>LMGCVAETPPRFTRTPVDQTGVSGGVASFICQATGDPRPKIVWNKKGKKVSNQRFEVIEFDDGSGSVLRIQPLRTPRDEAIYECVASNNVGEISVSTRLTVLREDQIPRGFPTIDMGPQLKVVERTRTATMLCAASGNPDPEITWFKDFLPVDTSNNNGRIKQLRSESIGGTPIRGALQIEQSEESDQGKYECVATNSAGTRYSAPANLYVRELREVRRVPPRFSIPPTNHEIMPGGSVNITCVAVGSPMPYVKWMLGAEDLTPEDDMPIGRNVLELNDVRQSANYTCVAMSTLGVIEAIAQITVKALPKPPGTPVVTESTATSITLTWDSGNPEPVSYYIIQHKPKNSEEPYKEIDGIATTRYSVAGLSPYSDYEFRVVAVNNIGRGPASEPVLTHHHHHH[2x];>QICPKRCVCQILSPNLATLCAKKGLLFVPPNIDRRTVELRLADNFVTNIKRKDFANMTSLVDLTLSRNTISFITPHAFADLRNLRALHLNSNRLTKITNDMFSGLSNLHHLILNNNQLTLISSTAFDDVFALEELDLSYNNLETIPWDAVEKMVSLHTLSLDHNMIDNIPKGTFSHLHKMTRLDVTSNKLQKLPPDPLFQRAQVLATSGIISPSTFALSFGGNPLHCNCELLWLRRLSREDDLETCASPPLLTGRYFWSIPEEEFLCEPPLITRHTHEMRVLEGQRATLRCKARGDPEPAIHWISPEGKLISNATRSLVYDNGTLDILITTVKDTGAFTCIASNPAGEATQIVDLHIIKLPHHHHHH[2x]

Type-IIa receptor protein tyrosine phosphatases (RPTPs) and neurexins are the two major presynaptic organizers. In mammals, the type-IIa RPTPs have three members, PTPδ, PTPσ, and LAR. These members possess a large extracellular domain (ECD) consisting of three immunoglobulin-like (Ig) domains and four to eight fibronectin type-III (Fn) domains, followed by a single transmembrane helix and a cytoplasmic domain harboring two protein tyrosine phosphatase (PTP) domains: the first PTP domain is active, while the second domain is inactive. SALM family proteins have five isoforms (SALM1–SALM5). Their ECDs share the same domain organization consisting of a leucine-rich repeat (LRR) domain, an Ig domain and an Fn domain with 35% amino-acid sequence identity. We determined the crystal structures of apo-SALM5 (LRR–Ig), and PTPδ (Ig1–Ig3)–SALM2 (LRR–Ig) and PTPδ (Ig1–Fn1)–SALM5 (LRR–Ig) complexes at 3.08, 3.16, and 4.18 Å resolutions, respectively.

In the PTPδ–SALM5 complex, the electron density of PTPδ Fn1 in one complex in the asymmetric unit was unclear, probably owing to the structural disorder. The interactions between PTPδ and SALM5 occur at three interfaces. The most extensive interface is formed between PTPδ Ig2 and SALM5 LRR. The second interface is formed between PTPδ Ig2 and SALM5 Ig. The third interface is formed between PTPδ Ig3 and SALM5 Ig. The meB-containing linker connecting Ig2 and Ig3 of PTPδ is stretched along SALM5, enabling PTPδ Ig3 to interact with SALM5 Ig. The meB insertion likely plays an important role in placing PTPδ Ig3 at the position favorable for the interaction with SALM5 Ig. A pseudo-C2 symmetric hydrogen bond network is extensively formed in the dimer interface. In the central region of the interface, Arg110 of one molecule hydrogen bonds with the main chains of His180 and Asn157 in another molecule (hereafter denoted by * after residue numbers), whereas Asn158 hydrogen bonds with Gln134*. The notable feature of the PTPδ–SALM5 complex is its 2:2 stoichiometry, which is required for its synaptogenic activity.> MSKDIKQVIEIAKKHNLFLKEETIQFNESGLDFQAVFAQDNNGIDWVLRLPRREDVMPRTKVEKQALDLVNKYAISFQAPNWIIYTEELIAYKKLDGVPAGTIDHNIGNYIWEIDINNVPELFHKSLGRVLAELHSIPSNKAAALDLVVHTPEEARMSMKQRMDAVRAKFGVGENLWNRWQAWLNDDDMWPKKTGLIHGDVHAGHTMIDKDANVTGLIDWTEAKVTDVSHDFIFNYRAFGEEGLEALILAYKEIGGYYWPKMKEHIIELNAAYPVSIAEFALVSGIEEYEQ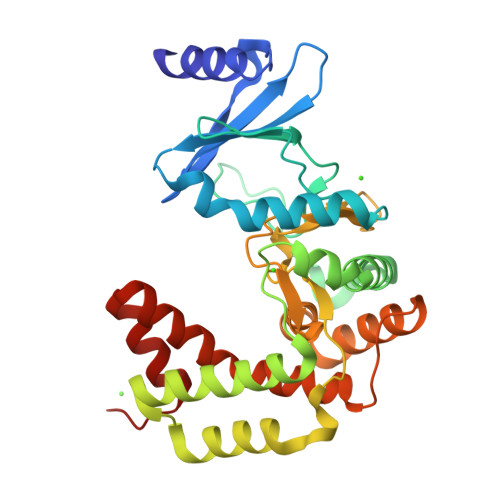MAKEALEVQGS>[4x]GSSTTFAARLNRLFDTVYPPGRGPHTSAEVIAALKAEGITMSAPY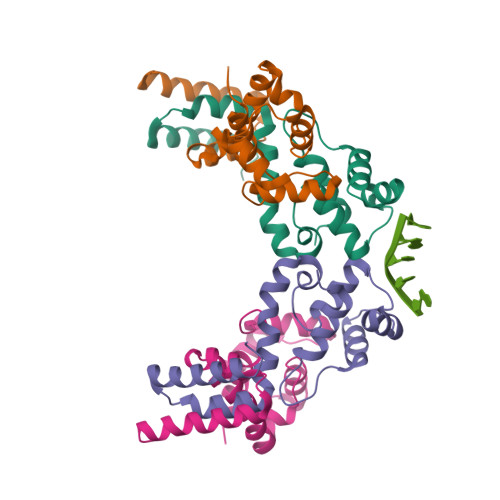LSQLRSGNRTNPSGATMAALANFFRIKAAYFTDDEYYEKLDKELQWLCTMRDDGVRRIAQRAHGLPSAAQQKVLDRIDELRRAEGIDA> DCSILELLKVKNQWREAFGEGHHRVQFGLELWKRFFDTHPEVK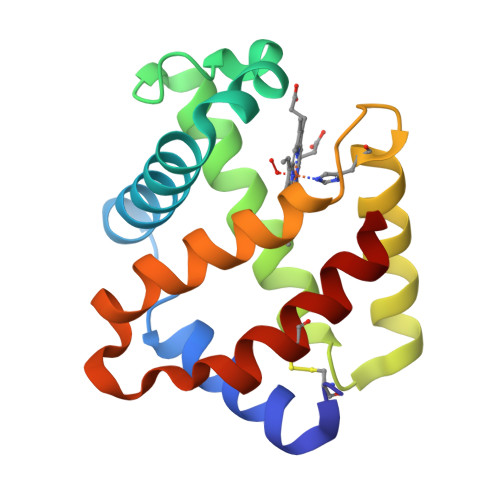GLFKGVNGDNIYSPEFAAHAERVLSGLDMTIGLLDDTNAFKAQVTHLHSQHVERSINPEFYEHFLGALLHVLPKYLGTKLDQDAWTKCFHTIADGIK Profilin is an ubiquitous cytoskeletal protein that interacts with several molecules, such as actin, proline-rich ligands, and phosphoinositides to perform several cellular functions. Profilin is also an important allergen present in pollen grains, food plants, and rubber tree, and it is considered a pan-allergen, because it is present in all eukaryotic cells and is therefore involved in allergic cross-reactions. In this work, we focus on the study of two plant pan-allergens, profilins from the rubber tree (rHev b 8) and maize (rZea m 12), in their monomeric and dimeric forms. Here we isolated the monomeric and dimeric species of the recombinant profilin allergens rHev b 8 and rZea m 12 and obtained their crystallographic 3D structures.

When the protein concentration was increased to 10 mg/mL, only one crystal of rHev b 8 was obtained, which contained two molecules in the asymmetric unit, as indicated by a Matthews coefficient of 3.06 Å3/Da and solvent content of 59.9%. This crystal belonged to the space group P32 and diffracted to a 2.8 Å resolution. In this study, we determined the tridimensional structure of a dimeric rHev b 8 stabilized by a disulfide bridge and compared it with the structures of the monomeric forms of the same allergen and that of rZea m 12. Interestingly, the dimeric structure of rHev b 8 displays a medium size interface stabilized through a disulfide bond that is formed between the two Cys13 residues of each monomer, which is conserved in all plant profilins. In addition, there are several hydrophobic and polar interactions between residues of α-helix 3 at the C-terminus and α-helix 1 at the N-terminal region (Fig. 2a right insert). From a functional point of view, the hydrophobic N- and C-terminal regions of the profilin structures are very important for their interaction with proline-rich proteins, such as kinases. This region is blocked when the dimer is formed; therefore, interactions with kinases could be limited. As observed in our dimer structure the interface blocks the kinase recognition region; therefore, we can suggest that the dimerization process might then have an auto-regulatory function for the members of the profilin family. Finally, we demonstrated that the dimeric form of rHev b 8 is more efficient than the monomeric form promoting significant degranulation in rat basophilic leukemia cells (RBL-2H3).

>MSWQAYVDDHLMCEIEGNHLSAAAIIGQDGSVWAQSANFPQFKSEEITGIMSDFHEPGTLAPTGLYIGGTKYMVIQGEPGAVIRGKKGPGGVTVKKTNQALIIGIYDEPMTPGQCNMIVERLGDYLIDQGY[2x]>[2x]KPRIDMHSHFFPRISEQEAAKFDANHAPWLQVSAKGDTGSIMMGKNNFAPVYQALWDPAFRIEEMDAQGVDVQVTCATPVMFGYTWEANKAAQWAERMNDFALEFAAHNPQRIKVLAQVP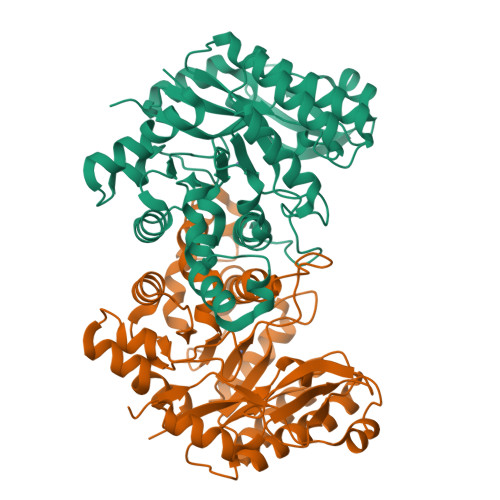LQDLDLACKEASRAVAAGHLGIQIGNHLGDKDLDDATLEAFLTHCANEDIPILVHPWDMMGGQRMKKWMLPWLVAMPAETQLAILSLILSGAFERIPKSLKICFGHGGGSFAFLLGRVDNAWRHRDIVREDCPRPPSEYVDRFFVDSAVFNPGALELLVSVMGEDRVMLGSDYPFPLGEQKIGGLVLSSNLGESAKDKIISGNASKFFNIN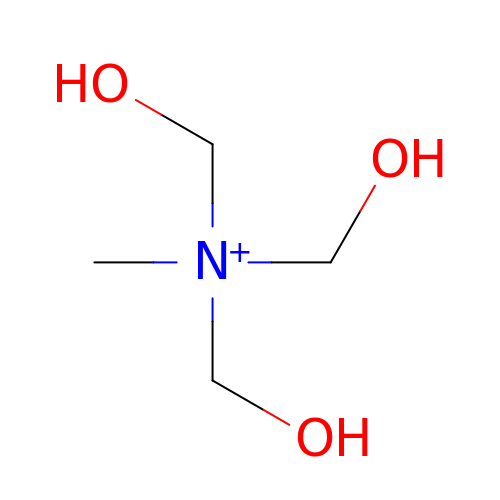TRIS-HYDROXYMETHYL-METHYL-AMMONIUM | C4 H12 N O3 | DRDCQJADRSJFFD-UHFFFAOYSA-N> MSFESKKPMRTWSHLAEMRKKPSEYDIVSRKLHYSTNNPDSPWEL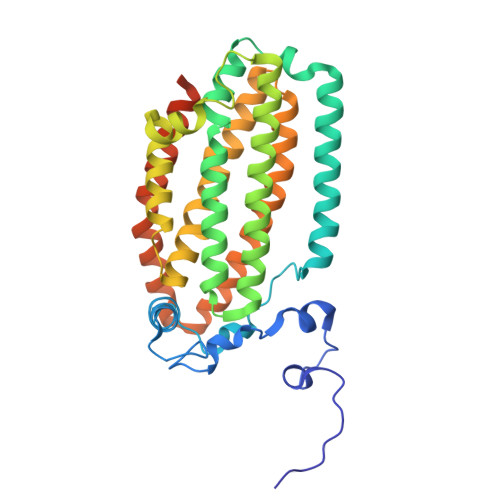SPDSPMNLWYKQYRNASPLKHDNWDAFTDPDQLVYRTYNLMQDGQESYVQSLFDQFNEREHDQMVREGWEHTMARCYSPLRYLFHCLQMSSAYVQQMAPASTISNCCILQTADSLRWLTHTAYRTHELSLTYPDAGLGEHERELWEKEPGWQGLRELMEKQLTAFDWGEAFVSLNLVVKPMIVESIFKPLQQQAWENNDTLLPLLIDSQLKDAERHSRWSKALVKHALENPDNHAVIEGWIEKWRPLADRAAEAYLSMLSSDILPAQYLERSTSLRASILTV> AKIGLFYGTQTGVTQTIAESIQQEFGGESIVDLNDIANADASDLNAYDYLIIGCPTWNVGELQSDWEGIYDDLDSVNFQGKKVAYFGAGDQVGYSDNFQDAMGILEEKISSLGSQTVGYWPIEGYDFNESKAVRNNQFVGLAIDEDNQP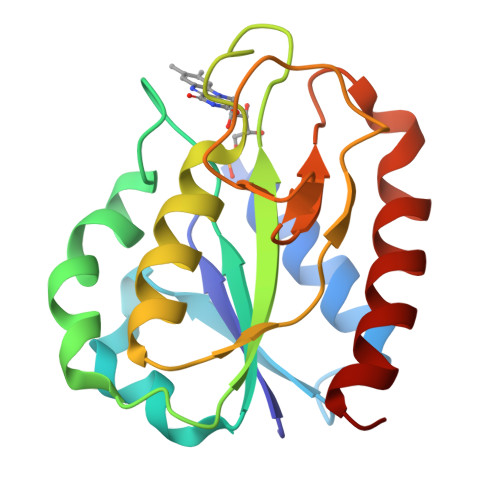DLTKNRIKTWVSQLKSEFGL> GPHMMVSDLKFAPSFQSFVDSSFFHELSRLKLDIFKLDSDEKALYTQLDLNQFTSNVLAISLRDDSFQKPDNDEHNIILKGYLLNFNTIELFKNCNKIQFIKEKGQELLQRGLENDLNEIISFYMISFADLKKYKFYYWICMPSFQSDGATYQIISSKVIASDSDISVSFIKQNVIIACVISGVIQKATPDNLKVCEKVVFKDFSHLKDIPSAVTKNILTVWSKLSPRETYTICFLRSDESSFEAEIIINNGNNPSLKVSGWEKNGLGKLAPKSIDLSSLMDP;> G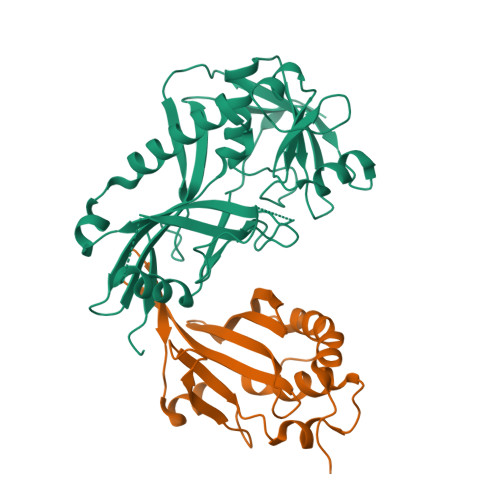PLGSMLTLPEYNEQIPNVRSLLTKWAKVERIQDVQDGLQLDVRLKTDTLLELHIYYDHVYHVPSIKFRLWSLDTEEDISSLRLLTLSDSELRSILNLGTFSVTLSTDMEMKSVYYYINNCDTDANVGSDVEHYLTRWISLYIRIFDLNFVP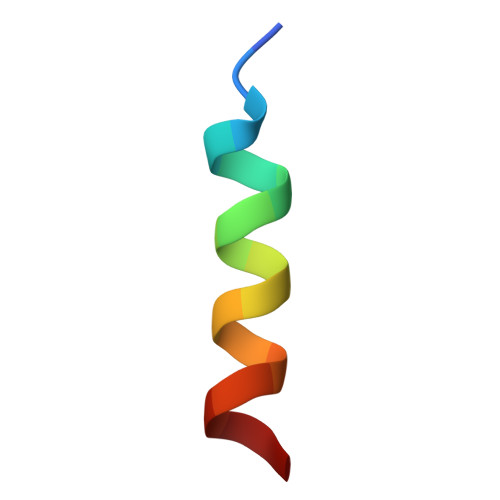> EDMFAKLKDKFFNEINK>[4x]MSNEIPKPVAPAPDILRCAYAELVVTDLAKSRNFYVDVLGLHVSYEDENQIYLRSFEEFIHHNLVLTKGPVAALKAMAFRVRTPEDVDKAEAYYQELGCRTERRKDGFVKGIGDALRVEDPLGFPYEFFFETTHVERLHMRYDLYSAGELVRLDHFNQVTPDVPRGRKYLEDLGFRVT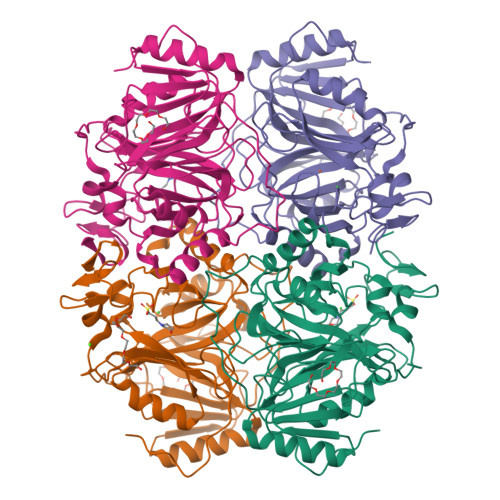EDIQDDEGTTYAAWMHRKGTVCDTALTGGNGPRLHHVAFSTHEKHNIIQICDKMGALRISDRIERGPGRHGVSNAFYLYILDPDNHRIEIYTQDYYTGDPDNPTITWNVHDNQRRDWWGNPVVPSWYTEASKVLDLDGNVQEIIERTDDSELEVTIGADGFSFTRAGDEDGSYHGQASKGFKLGNQL PURVALANOL B | C20 H25 Cl N6 O3 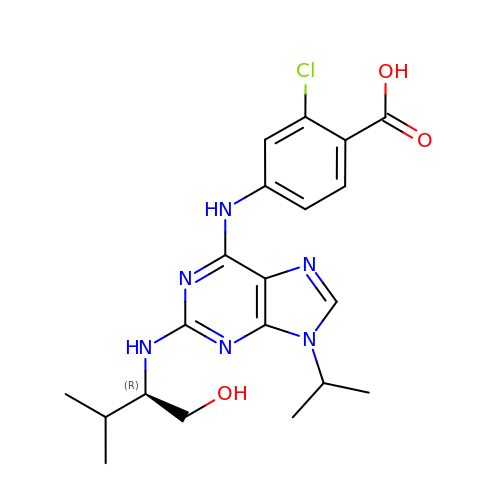| ZKDXRFMOHZVXSG-HNNXBMFYSA-N KSHV is a member of the gammaherpesvirus subfamily and is the causative agent of several devastating diseases, including Kaposi’s sarcoma, primary effusion lymphoma, and multicentric Castleman’s disease. Glycoprotein B (gB) is the fusogen responsible for the physical action of membrane fusion and is conserved across all herpesviruses. As a class III fusion protein, gB undergoes a conformational change from a prefusion state to a postfusion state that draws the host and viral envelopes together to induce fusion. Here, we report the first structure of the KSHV gB ectodomain determined by single-particle cryogenic electron microscopy (cryoEM).

To alleviate this issue, we truncated the sequence and determined the structure of the soluble ectodomain of KSHV gB (amino acid residues 1–687). Of the homologous mutation sites at the DIII central helix, D470P was selected for structural determination for its expression level and charged sidechain. The structure of KSHV gB was determined at 3.3 Å resolution by single particle cryoEM. The gB structure was reconstructed as a homotrimer with C3 symmetry aligned along the long edge. KSHV gB ectodomain exhibits an elongated rod-shaped architecture with dimensions approximately 70 Å by 70 Å by 170 Å, consistent with the postfusion conformation observed in other herpesvirus fusion proteins, such as those from HSV-1, VZV, HCMV, and EBV. The KSHV gB follows a canonical postfusion domain organization of the class III fusion protein, with its core comprising three β-strand-rich modular domains (DI, DII, and DIV) and a long three-helix bundle of DIII. Of the 13 hypothetical glycosylation sites per protomer based on consensus sequence in KSHV gB, 10 sites displayed the densities for glycan chains. Notably, the glycan at N179 showed an extended sugar chain density, corresponding to up to eight sugar molecules, including two branching points. In general, the folds of each domain are nearly identical between herpesvirus species, but we observe that a loop in DI of KSHV gB at residues 252–270 deviates greatly from all currently known gB structures. The DIV trimer region exhibits a rotational movement around the three-fold symmetry axis, while the remaining ectodomain (DI-DIII, DV) remains largely static.

>[3x]ASGPKSVDFYQFRVCSASITGELFRFNLEQTCPDTKDKYHQEGILLVYKKNIVPHIFKVRRYRKIATSVTVYRGLTESAITNKYELPRPVPLYEISHMDSTYQCFSSMKVNVNGVENTFTDRDDVNTTVFLQPVEGLTDNIQRYFSQPVIYAEPGWFPGIYRVRTTVNCEIVDMIARSAEPYNYFVTSLGDTVEVSPFCYNESSCSTTPSNKNGLSVQVVLNHTVVTYSDRGTSPTPQNRIFVETGAYTLSWASESKTTAVCPLALWKTFPRSIQTTHEDSFHFVANEITATFTAPLTPVANFTDTYSCLTSDINTTLNASKAKLASTHVPNGTVQYFHTTGGLYLVWQPMSAINLTHAQGDRGNPTSSPPPSASPVTTSASRRKRRSASTAAAGGGGSTDNLSYTQLQFAYDKLRPGINQVLEELSRAWCREQVRDNLMWYELSKINPTSVMTAIYGRPVSAKFVGDAISVTECINVDQSSVNIHKSLRTNSKDVCYARPLVTFKFLNSSNLFTGQLGARNEIILTNNQVETCKDTCEHYFITRNETLVYKDYAYLRTINTTDISTLNTFIALNLSFIQNIDFKAIELYSSAEKRLASSVFDLETMFREYNYYTHRLAGLREDLDNTIDMNKE>[2x]GSHMEPPPKLVLDLERLATVPAEKAGPLQRYAATIQSQRGDYNGKVLSIRQDDLRTLAVIYDQSPSVLTEQLISWGVLDADARRAVASHDEL

Here, we report that c-di-GMP can assemble into a tetramer that mediates the effective dimerization of a transcription factor, BldD, which controls the progression of multicellular differentiation in sporulating actinomycete bacteria. BldD is an 18 kDa DNA-binding protein consisting of two distinct domains connected by a flexible linker. BldD sits at the top of the regulatory cascade controlling development, serving to repress expression of sporulation genes during vegetative growth (den Hengst et al., 2010). Specifically, structural and biochemical analyses show that the second messenger c-di-GMP activates BldD DNA binding by driving a unique form of dimerization that is mediated by a tetrameric form of c-di-GMP.

To elucidate the molecular basis for c-di-GMP recognition and binding by the BldD CTD and to gain insight into how this interaction may elicit developmental signaling, we determined structures of the S. venezuelae BldD CTD (residues 80–166) and S. coelicolor BldD CTD (residues 80–167) in complex with c-di-GMP. Three S. venezuelae BldD C-domain-(c-di-GMP) structures and one S. coelicolor BldD C-domain-(c-di-GMP) structure were determined to resolutions of 1.95 Å, 2.33 Å, 1.75 Å, and 2.25 Å, respectively (see Extended Experimental Procedures and Tables S1 and S2). Further, BldD from S. coelicolor and S. venezuelae contain an identical DBD and differ by only two residues in the DBD-CTD linker and five residues in the CTD, suggesting that BldD function is broadly conserved between the two species. The BldD CTD uses a previously unseen mode of c-di-GMP binding in which two noninteracting CTDs are glued together by a c-di-GMP tetramer composed of two interlocked c-di-GMP dimers. The BldD CTD interacts with c-di-GMP using two contiguous surface motifs, herein called motif 1 and motif 2, which are located between the two β-α-α repeats. Motif 1 is composed of residues 114–116 (RGD) and motif 2 is composed of residues 125–128 (RQDD). The combined motifs from two CTD subunits provide ideal shape and electrostatic complementarity for encasing the unusual cage-like c-di-GMP tetramer. Further, mutagenesis of either BldD motif 1 or motif 2 abolishes c-di-GMP binding in DRaCALA assays, confirming that, unlike I-site c-di-GMP binding, both motifs 1 and 2 in BldD are required to construct the complete binding site for the tetrameric c-di-GMP complex. Overall, these data demonstrate unequivocally that c-di-GMP binds the CTD with a stoichiometry of four c-di-GMP molecules per CTD dimer, concordant with our structures. Notably, the identical CTD dimer-(c-di-GMP) tetramer structure was seen in multiple crystal forms.>[2x]GPAMASKSPSEEVYPVKAFGLAAKDSSGLFSPFNFSRRATGEHDVQLKVLYCGTCQYDREMSKNKFGFTSYPYVLGHEIVGEVTEVGSKVQKFKVGDKVGVASIIETCGKCEMCTNEVENYCPEAGSIDSNYGACSNIAVINENFVIRWPENLPLDSGVPLLCAGITAYSPMKRYGLDKPGKRIGIAGLGGLGHVALRFAKAFGAKVTVISSSLKKKREAFEKFGADSFLVSSNPEEMQGAAGTLDGIIDTIPGNHSLEPLLALLKPLGKLIILGAPEMPFEVPAPSLLMGGKVMAASTAGSMKEIQEMIEFAAEHNIVADVEVISIDYVNTAMERLDNSDVRYRFVIDIGNTLKSN

Crystal structures of THAS (here referred to as THAS1), a second representative THAS (Cr_021691, THAS2) and the structure of the promiscuous homologue (Cr_032583b, HYS) were solved and mutants revealed key residues that control the stereochemistry of the product profiles. The HYSs perform a single, chemically straightforward reduction reaction that immediately neutralizes the reactivity of strictosidine aglycone/cathenamine. The biological unit is an elongated homodimer, with each subunit divided into a substrate and cofactor-binding domain; the latter also being responsible for forming the dimer interface. The active site cavities of the HYSs are framed by helix α2, the catalytic zinc coordination sphere, and loops 1 and 2, with the NADP(H) co-substrate binding at the base of the active site.

Structures were obtained for THAS1 and THAS2 with NADP+ bound (THAS1, 1.05 Å resolution; THAS2, 2.10 Å resolution) and in apo form (THAS1, 2.25 Å resolution; THAS2, 2.05 Å resolution), while HYS could only be crystallized in the apo form (2.25 Å resolution). In both THAS1 and THAS2, a network of amino acids holds NADP+ in place. Most notably, Glu59 of THAS1 anchors NADP(H) through a bidentate interaction with both ribose hydroxyls, with His59 playing a comparable role in SAD, although here the interaction is with the 3′ OH only. The proximal zinc of THAS1 is ∼2 Å further away from the cofactor relative to SAD and thus may play no direct role in catalysis. However, it may have a function in maintaining the tertiary structure since three of the liganding residues are in the substrate-binding domain and the fourth is in the cofactor-binding domain. SAD/CAD utilize an active site serine that protonates the alkoxide that results from reduction of the aldehyde substrate; this serine is replaced with a tyrosine residue in THAS1 (Tyr56) and HYS (Tyr53). Interestingly, a non-proline cis-peptide is present in the THAS1-NADP+ and HYS apo structures. Closer inspection of this region in THAS1 shows that when this bond is in the trans conformation, the side chain of Asp340 is projected into the cofactor-binding site such that it would prevent NADPH binding. In silico docking with THAS1 positions cathenamine between the nicotinamide of the NADP+ and Tyr56, which is located on helix α2. THAS1 loop 1 contains Phe65 that also projects into the active site and may interact with the aromatic cathenamine substrate.>GPGSVRVVRGRGLLRAVLDRPERRNPIDAGLLTSLARALDQAESDQDCRVFVLSSTGEDF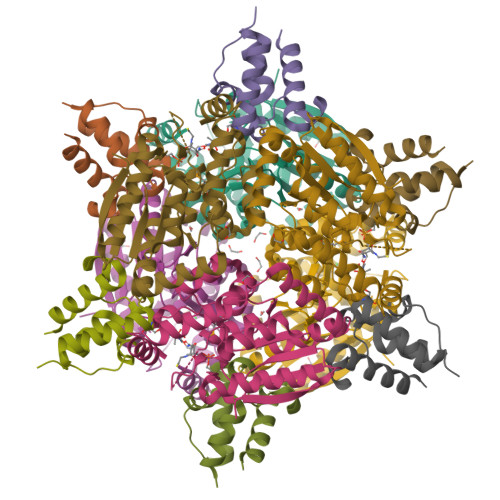CAGTDLSGGDPAPEPLPDGAELPYWTLLERLTRSPLATVAVVDGRATAGGVGLAAACDLVLAGERARFRLTEVLAGLVPAMALPFVARRTGEQRAFAATLRAEEFDAGAAHRVGLADLAGPRAEDLLPPVLAGLGRTDRSTTAALKEYRARLFPRDARLGHDASRLLIERFAAPGTGQLLARLREAGAAA[2x];>[2x]GPGSAVAVDPAPVARALREELARTLYCEPGDIDDEASFNTLGLDSILGVEFVAFVNQTYGLDEKAGILYDHPSLAALSRHVAGRAAPV> AASTLDEIMKRGTLRVGTDADYKPFSFKDKNGQYTGFDIDLAKALAKELGVKVEFVPTTWDGIIPALQTGKFDIVMSGMTITPERKKKVDFSDPYMTAGQTILVKKDNADKIKSFEDLNKPD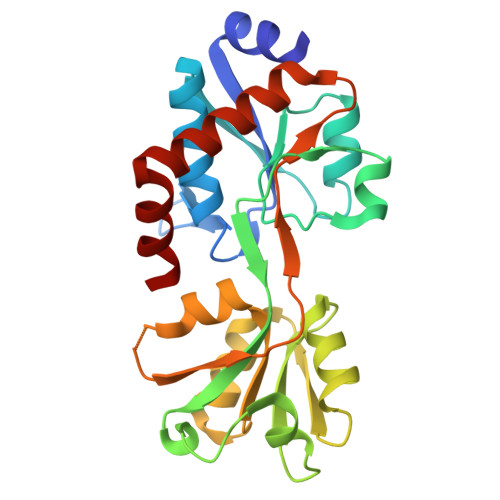VKVAVQLGTTSEQAAKEFLPKAKIRTFENNAEAFQEVVSGRADAMVTDSPVAAYYAKKNPGLAVVVVDEPFTHEPLGFAIRKGDPELLNWVNNWLKQMKKDGTYDKLYEKWFK>[2x]DYKDDDDKMTNLPEHQSSPTEQSSAEVKKIPTMIEGFDDISHGGLPQGRTTLVSGTSGTGKTLF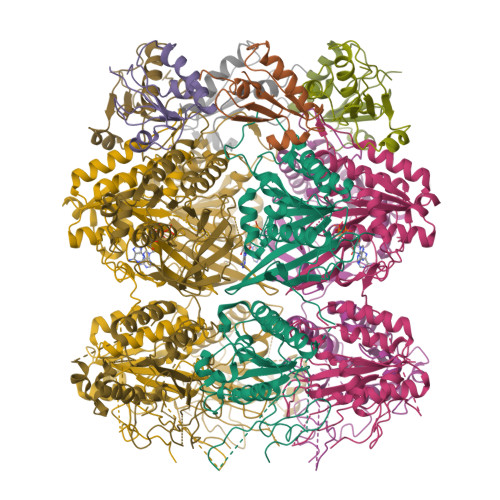AVQFLYNGITIFNEPGIFVTFEESPQDIIKNALSFGWNLQSLIDQGKLFILDASPDPDGQEVAGDFDLSALIERIQYAIRKYKATRVSIDSVTAVFQQYDAASVVRREIFRLAFRLKQLGVTTIMTTERVDEYGPVARFGVEEFVSDNVVILRNVLEGERRRRTVEILKLRGTTHMKGEYPFTINNGINIFPLGAMRLTQRSSNVRVSSGVKTLDEMCGGGFFKDSIILATGATGTGKTLLVSKFLETGCQQGERALLFAYEESRAQLSRNASSWGIDFEELERRGLLRIICAYPESAGLEDHLQIIKSEIADFKPSRVAIDSLSALARGVSNNAFRQFVIGVTGFAKQEEITGFFTNTTDQFMGSNSITESHIETITDTILLLQYVEIRGEMSRAINVFKMRGSWHDKGIREYVITEKGAEIRDSFRNFEGIISGTPTRISVDEKTELARIAKGMQDLESE;>[2x]MAPLRKTAVLKLYVAGNTPNSVRALKTLNNILEKEFKGVYALKVIDVLKNPQLAEEDKILATPTLAKVLPPPVRRIIGDLSNREKVLAGLDLLAEEIGD>AQYEDGKQYTTLEKPVAGAPQVLEFFSFFCPHCYQFEE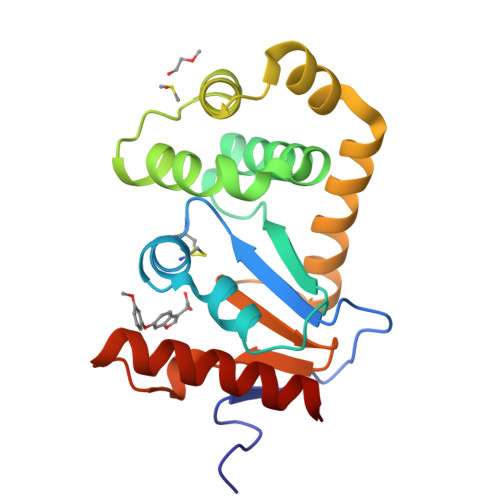VLHISDNVKKKLPEGVKMTKYHVNFMGGDLGKDLTQAWAVAMALGVEDKVTVPLFEGVQKTQTIRSASDIRDVFINAGIKGEEYDAAWNSFVVKSLVAQQEKAAADVQLRGVPAMFVNGKYQLNPQGMDTSNMDVFVQQYADTVKYLSEKK[2x]> MELKHSISDYTEAEFLQLVTTI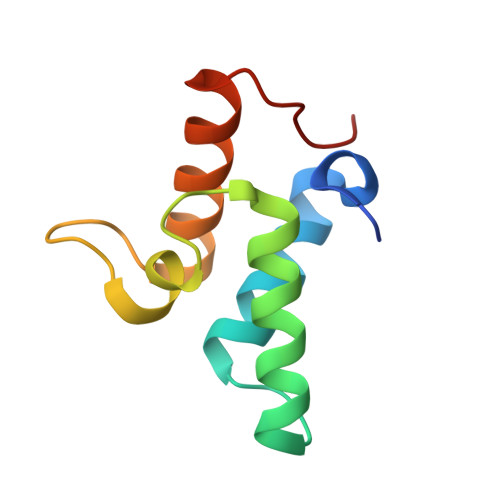CNADTSSEEELVKLVTHFEEMTEHPSGSDLIYAPKEGDDDSPSGIVNTVKQWRAANGKSGFKQG> MKKIIYIATIGITLLTTSCDD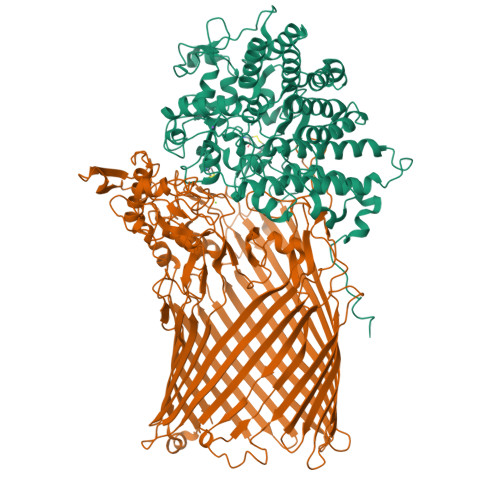FLDRQVPQGIVTGDQIASPEYVDNLVISAYAIWATGDDINSSFSLWNYDVRSDDCYKGGSGTEDGGVFNALEISKGINTTDWNINDIWKRLYQCITRANTALQSLDQMDEKTYPLKNQRIAEMRFLRGHAHFMLKQLFKKIVIVNDENMEPDAYNELSNTTYTNDEQWQKIADDFQFAYDNLPEVQIEKGRPAQAAAAAYLAKTYLYKAYRQDGADNALTGINEEDLKQVVKYTDPLIMAKGGYGLETDYSMNFLPQYENGAESVWAIQYSINDGTYNGNLNWGMGLTTPQILGCCDFHKPSQNLVNAFKTDSQGKPLFSTYDNENYEVATDNVDPRLFHTVGMPGFPYKYNEGYIIQKNDDWSRSKGLYGYYVSLKENVDPDCDCLKKGSYWASSLNHIVIRYADVLLMRAEALIQLNDGRITDAISLINEVRSRAAGSTMLIFNYKEDYGVNFKVTPYDLKAYAQDEAMKMLKWERRVEFGMESSRFFDLVRWGEAKDVINAYYVTEASRCSIYKNAGFTENKNEYLPVPFEQISASNGNYTQNFGWHHHHHH;> MPGIMKNKKLLCSVCFLFAFMSALWGQNITVKGNVTSKTDGQPIIGASVVETTATTNGTITDFDGNFTLSVPVNSTLKITYIGYKPVTVKAAAIVNVLLEEDTQMVDEVVVTGYTTQRKADLTGAVSVVKVDEIQKQGENNPVKALQGRVPGMNITADGNPSGSATVRIRGIGTLNNNDPLYIIDGVPTKAGMHELNGNDIESIQVLKDAASASIYGSRAANGVIIITTKQGKKGQIKINFDASVSASMYQSKMNVLNTEQYGRAMWQAYVNDGENPNGNALGYAYNWGYNADGNPVLYGMTLSKYLDSKNTMPVADTDWFDEITRTGVIQQYNLSVSNGSEKGSSFFSLGYYKNLGVIKDTDFDRFSARMNSDYKLIDDILTIGQHFTLNRTSEVQAPGGIIETALDIPSAIPVYASDGSWGGPVGGWPDRRNPRAVLEYNKDNRYTYWRMFGDAYVNLTPFKGFNLRSTFGLDYANKQARYFTYPYQEGTQTNNGKSAVEAKQEHWTKWMWNAIATYQLEVGKHRGDVMIGMELNREDDSHFSGYKEDFSILTPDYMWPDAGSGTAQAYGAGEGYSLVSFFGKMNYSYADRYLLSLTLRRDGSSRFGKNHRYATFPSVSLGWRITQENFMKELTWLDDLKLRASWGQTGNQEISNLARYTIYAPNYGTTDSFGGQSYGTAYDITGSNGGGVLPSGFKRNQIGNDNIKWETTTQTNVGIDFSLFKQSLYGSLEYYYKKATDILTEMAGVGVLGEGGSRWINSGAMKNQGFEFNLGYRNKTAFGLTYDLNGNISTYRNEILELPETVAANGKFGGNGVKSVVGHTYGAQVGYIADGIFKSQDEVDNHATQEGAAVGRIRYRDIDHNGVIDERDQNWIYDPTPSFSYGLNIYLEYKNFDLTMFWQGVQGVDIISDVKKKSDFWSASNVGFLNKGTRLLNAWSPTNPNSDIPALTRSDTNNEQRVSTYFVENGSFLKLRNIQLGYTVPAVISKKMRMDRLRFYCSAQNLLTIKSKNFTGEDPENPNFSYPIPVNITFGLNIGF> MSDGAVQPDGGQPAVRNERATGSGNGSGGGGGGGSGGVGISTGTFNNQTEFKFLENGWVYITANSSRLVHLNMPESENYRRVVVNNMDKTAVNGNMALDDIHAEIVTPWSLVDANAW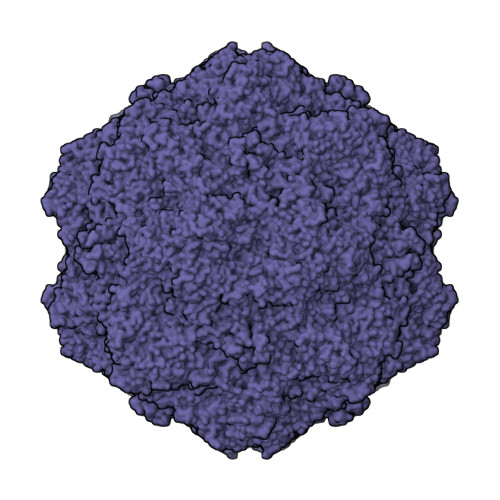GVWFNPGDWQLIVNTMSELHLVSFEQEIFNVVLKTVSESATQPPTKVYNNDLTASLMVALDSNNTMPFTPAAMRSETLGFYPWKPTIPTPWRYYFQWDRTLIPSHTGTSGTPTNIYHGTDPDDVQFYTIENSVPVHLLRTGDEFATGTFFFDCKPCRLTHTWQTNRALGLPPFLNSLPQSEGDTNFGDIGVQQDKRRGVTQMGNTNYITEATIMRPAEVGYSAPYYSFEASTQGPFKTPIAAGRGGAQTDENQAADGNPRYAFGRQHGQKTTTTGETPERFTYIAHQDTGRYPEGDWIQNINFNLPVTNDNVLLPTDPIGGKTGINYTNIFNTYGPLTALNNVPPVYPNGQIWDKEFDTDLKPRLHVNAPFVCQNNCPGQLFVKVAPNLTNQYDPDASANMSRIVTYSDFWWKGKLVFKAKLRASHTWNPIQQMSINVDNQFNYVPSNIGGMKIVYEKSQLAPRKLY>GGSGERKISRIHLVSEPSITHFLQVSWEKT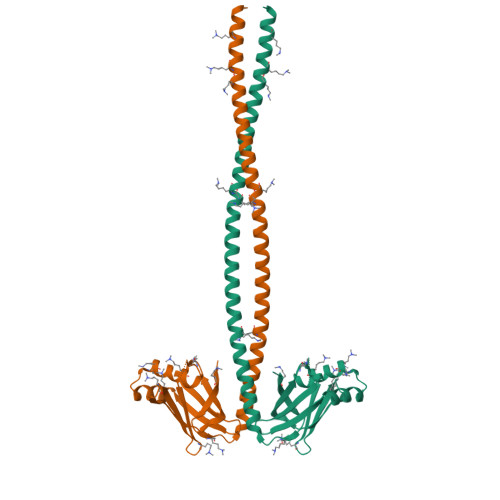LESGFVITLTDGHSAWTGTVSESEISQEADDMAMEKGKYVGELRKALLSGAGPADVYTFNFSKESCYFFFEKNLKDVSFRLGSFNLEKVENPAEVIRELICYCLDTTAENQAKNEHHLRVVDSLQTSLDAETRSRNEALRVKKKMEGDLNEMEIQLSHANRMAAEAQKQVKSLQSLLKDTQIQL[2x]> MAEKQKHDGRVKIGHYVLGDTLGVGTFGKVKIGEHQLTGHKVAVKILNRQKIRSLDVVGKIKREIQNLKLFRHPHIIKLYQVISTPT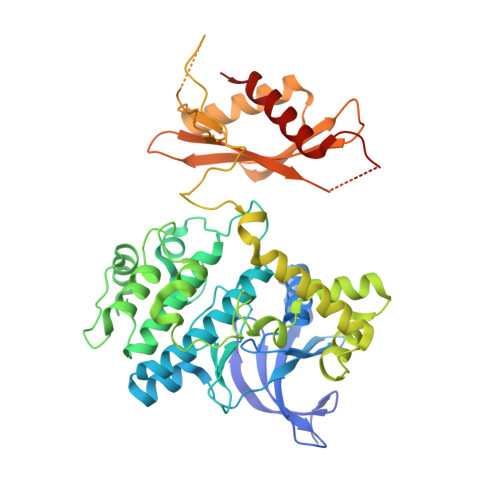DFFMVMEYVSGGELFDYICKHGRVEEMEARRLFQQILSAVDYCHRHMVVHRDLKPENVLLDAHMNAKIADFGLSNMMSDGEFLRTSCGSPNYAAPEVISGRLYAGPEVDIWSCGVILYALLCGTLPFDDEHVPTLFKKIRGGVFYIPEYLNRSVATLLMHMLQVDPLKRATIKDIREHEWFKQDLPSYLFPEDPSYDANVIDDEAVKEVCEKFECTESEVMNSLYSGDPQDQLAVAYHLIIDNRRIMNQASEFYLASSPPSGSFMDDSAMHIPPGLKPHPERMPPLIADSPKARCPLDALNTTKPKSLAVKKAKWHLGIRSQSKPYDIMAEVYRAMKQLDFEWKVVNAYHLRVRRKNPVTGNYVKMSLQLYLVDNRSYLLDFKSIDDEVVEQRSGSSTPQRSCSAAGLHRPRSSFDSTTAESHSLSGSLTGSLTGSTLSSVSPRLGSHTMDFFEMCASLITTLAR>[16x]MIPARFAGVLLALALILPGTLCAEGTRGRSSTARCSLFGSDFVNTFDGSMYSFAGYCSYLLAGGCQKRSFSIIGDFQNGKRVSLSVYLGEFFDIHLFVNGTVTQGDQRVSMPYASKGLYLETEAGYYKLSGEAYGFVARIDGSGNFQVLLSDRYFNKTCGLCGNFNIFAEDDFMTQEGTLTSDPYDFANSWALSSGEQWCERASPPSSSCNISSGEMQKGLWEQCQLLKSTSVFARCHPLVDPEPFVALCEKTLCECAGGLECACPALLEYARTCAQEGMVLYGWTDHSACSPVCPAGMEYRQCVSPCARTCQSLHINEMCQERCVDGCSCPEGQLLDEGLCVESTECPCVHSGKRYPPGTSLSRDCNTCICRNSQWICSNEECPGECLVTGQSHFKSFDNRYFTFSGICQYLLARDCQDHSFSIVIETVQCADDRDAVCTRSVTVRLPGLHNSLVKLKHGAGVAMDGQDVQLPLLKGDLRIQHTVTASVRLSYGEDLQMDWDGRGRLLVKLSPVYAGKTCGLCGNYNGNQGDDFLTPSGLAEPRVEDFGNAWKLHGDCQDLQKQHSDPCALNPRMTRFSEEACAVLTSPTFEACHRAVSPLPYLRNCRYDVCSCSDGRECLCGALASYAAACAGRGVRVAWREPGRCELNCPKGQVYLQCGTPCNLTCRSLSYPDEECNEACLEGCFCPPGLYMDERGDCVPKAQCPCYYDGEIFQPEDIFSDHHTMCYCEDGFMHCTMSGVPGSLLPDAVLSSPLSHASASLSCRPPMVKLVCPADNLRAEGLECAKTCQNYDLECMSMGCVSGCLCPPGMVRHENRCVALERCP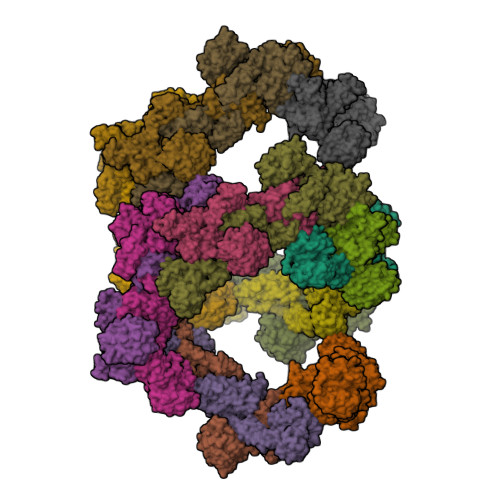CFHQGKEYAPGETVKIGCNTCVCRDRKWNCTDHVCDATCSTIGMAHYLTFDGLKYLFPGECQYVLVQDYCGSNPGTFRILVGNKGCSHPSVKCKKRVTILVEGGEIELFDGEVNVKRPMKDETHFEVVESGRYIILLLGKALSVVWDRHLSISVVLKQTYQEKVCGLCGNFDGIQNNDLTSSNLQVEEDPVDFGNSWKVSSQCADTRKVPLDSSPATCHNNIMKQTMVDSSCRILTSDVFQDCNKLVDPEPYLDVCIYDTCSCESIGDCACFCDTIAAYAHVCAQHGKVVTWRTATLCPQSCEERNLRENGYECEWRYNSCAPACQVTCQHPEPLACPVQCVEGCHAHCPPGKILDELLQTCVDPEDCPVCEVAGRRFASGKKVTLNPSDPEHCQICHCDVVNLTCEACQEPGGLVVPPTDAPVSPTTLYVEDISEPPLHDFYCSRLLDLVFLLDGSSRLSEAEFEVLKAFVVDMMERLRISQKWVRVAVVEYHDGSHAYIGLKDRKRPSELRRIASQVKYAGSQVASTSEVLKYTLFQIFSKIDRPEASRIALLLMASQEPQRMSRNFVRYVQGLKKKKVIVIPVGIGPHANLKQIRLIEKQAPENKAFVLSSVDELEQQRDEIVSYLCDLAPEAHHHHHH>[2x]APVWGCASTRGRSAEMEDASAAVPRFADVPVRLLASRRDLDALGLDADALRLPAHLFGVFDGHGGAEVANYCRERIHVVLSAALARLGKNLGEMGEVDMKEHWDDVFTKCFQRVDDEVSGRVTRVVNGGGEVRSEPVTAENVGSTAVVALVCSSHVVVANCGDSRIVLCRGKEPVALSIDHKPDRKDERARIEAQGGKVIQWNGYRVSGILAMSRSIGDRYLKPFVIPKPEVMVVPRAKDDDCLILASDGLWDVVSNEEACKVARRQILLWHKNNGAASPLSDEGEGSTDPAAQAAADYLMRLALKKGSEDNITVIVVDLKPRKKLKN;>[2x]ETEYVRRFHRHEPRDHQCSSAVAKHIKAPVHLVWSLVRRFDQ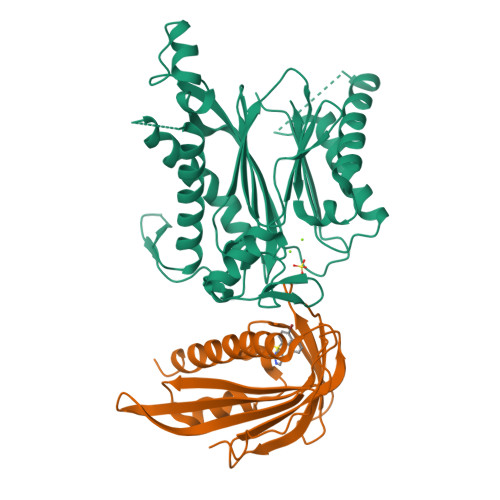PQLFKPFVSRCEMKGNIEIGSVREVNVKSGLPATRSTERLELLDDNEHILSVRFVGGDHRLKNYSSILTVHPEVIDGRPGTLVIESFVVDVPEGNTKDETCYFVEALLKCNLKSLAEVSERLVVKDQTEPLDR> GSRPGPASQLPRFVRVNTLKTCSDDVVDYFKRQGFSYQGRA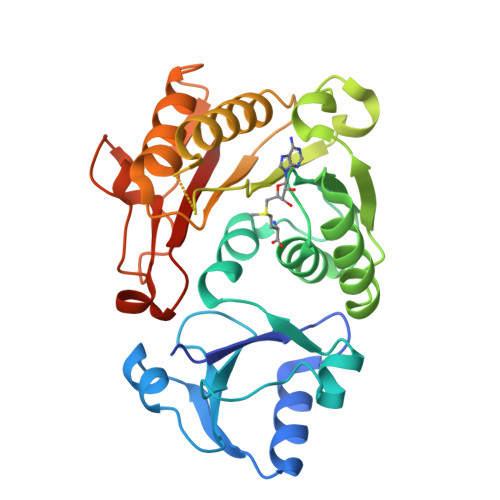SSLDDLRALKGKHFLLDPLMPELLVFPAQTDLHEHPLYRAGHLILQDRASCLPAMLLDPPPGSHVIDACAAPGNKTSHLAALLKNQGKIFAFDLDAKRLASMATLLARAGVSCCELAEEDFLAVSPSDPRYHEVHYILLDPSCSGSGMPSRQLEEPGAGTPSPVRLHALAGFQQRALCHALTFPSLQRLVYSTCSLCQEENEDVVRDALQQNPGAFRLAPALPAWPHRGLSTFPGAEHCLRASPETTLSSGFFVAVIERVEVPRRARG>[4x]MEEAYLALGKKILEEGHFKEDRTGTGTYSLFGYQMRFDLAKGFPLLTTKRVPFGLIKSELLWFLKGDTNIRYLLERNNHIWDEWAFERYVKSADYQGPDMTDFGHRVLQDPAFAEQYKEEHQKFCDAILNDAEFAEKYGELGNIYGAQWRHWETKDGSFIDQLANVIEMIKTNPDSRRLIVSAWNPEDVPSMALPP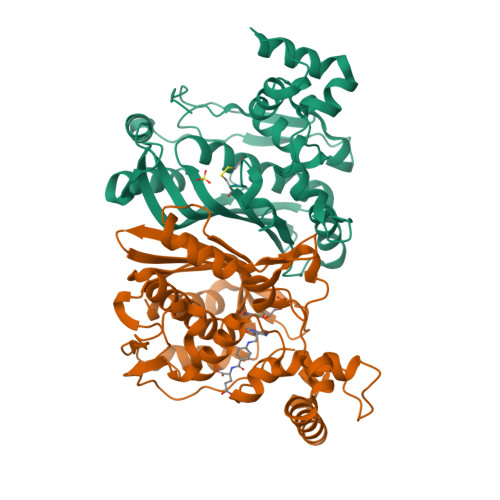CHTMFQFYVNEGKLSCQLYQRSADVFLGVPFNIASYALLTHLIAHETGLEVGEFVHTLGDAHLYQNHVEQMQEQLSREVRSFPTLVLNPDKASVFDFDMEDIKVEGYDPHPTIKAPIAV MALACHITE GREEN | C23 H25 N2 | 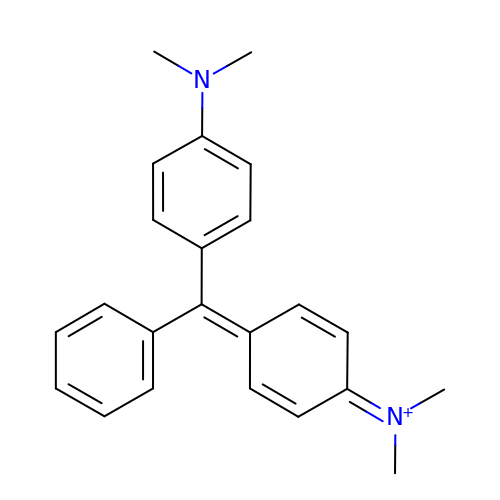VFCNQNZNPKRXIT-UHFFFAOYSA-N>[2x]MKNERIEKLQESWELDERWEGITRPYSAEDVIRLRGSIDIEHTLARRGAEKLWTSLHTEDYINALGALTGNQAMQQVKAGLKAIYLSGWQVAADANLSGHMYPDQSLYPANSVPAVVKRINQTLQRADQIQHMEGSDDTDYFVPIVADAEAG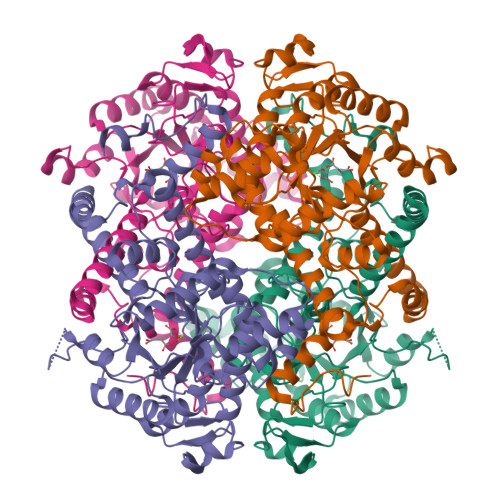FGGQLNVFELMKGMIEAGASGVHFEDQLSSEKKCGHLGGKVLLPTQTAVRNLISARLAADVMGVPTIIVARTDADAADLITSDIDPVDKAFITGERTPEGFYRTNAGLDQAIARGLAYAPYADLVWCETSEPNLEDAKRFADAIHKEHPGKLLAYNCSPSFNWKQKLDEKAIASFQKEIASYGYKFQFVTLAGFHSLNYGMFELARGYKERGMAAYSELQQAEFAAEKHGYSATRHQREVGTGYFDEVAQVITGGTSSTTALKGSTEEAQFTKLEHHHHHH>SNDCVLDVMHAIYQQNKEHFQDECTKLLVGNIVITRYNNRTYRIDDVDWNKTPKDSFTMSDGKEITFLEYYSKNYGITVKEEDQPLLIHRPSERQD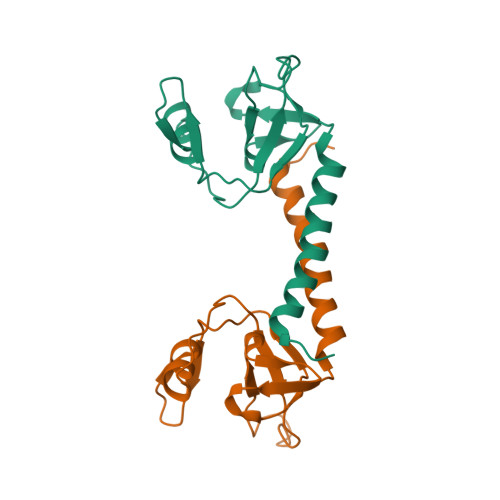NHGMLLKGEILLLPELSFMTGIPEKMKKDFRAMKDLAQQINLSP[4x]>[2x]MVVMIKLRDELGTATTDSAQKILLLGSGELGKEIAIEAQRLGVEVVAVDRYANAPAMQVAHRSYVGNMMDKDFLWSVVEREKPDAIIPEIEAINLDALFEFEKDGYFVVPNARATWIAMHRERLRETLVKEAKVPTSRYMYATTLDELYEACEKIGYPCHTKAIMSSSGKGSYFVKGPEDIPKAWEEAKTKARGSAEKIIVEEHIDFDVEVTELAVRHFDENGEIVTTFPKPVGHYQIDGDYHASWQP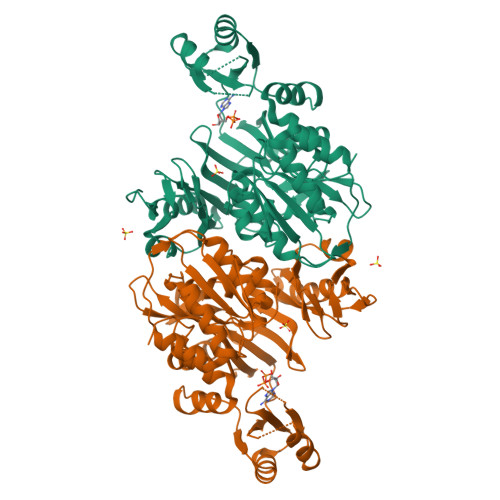AEISEKAEREVYRIAKRITDVLGGLGIFGVEMFVKGDKVWANEVSPRPHDTGMVTLASHPPGFSEFALHLRAVLGLPIPGEWVDGYRLFPMLIPAATHVIKAKVSGYSPRFRGLVKALSVPNATVRLFGKPEAYVGRRLGIALAWDKDVEVAKRKAEMVAHMIELRTRSSDWHDQNYEKRKHLLR>MSNQLFDAYFTAPAMREIFSDRGRLQGMLDFEAALARAEASAGLVPHSAVAAIEAACQAERYDTGALANAIATAGNSAIPLVKALGKVIATGVPEAERYVHLGATSQDAMDTGLVLQLRDALDLIEADLGKLADTLSQQALKHADTPLVGRTWLQHATPVTLGMKLAGVLGALTRHRQRLQELRPRLLVLQFGGASGSLAALGSKAMPVAEALAEQLKLTLPEQPWHTQRDRLVEFASVLGLVAGSLGKFGRDISLLMQTEAGEVFEPSAPGKGGSSTMPHKRNPVGAAVLIGAATRVPGLLSTLFAAMPQEHERSLGLWHAEWETLPDICCLVSGALRQAQVIAEGMEVDAARMRRNLDLTQGLVLAEAVSIVLAQRLGRDRAHHLLEQCCQRAVAEQRHLRAVLGDEPQVSAELSGEELDRL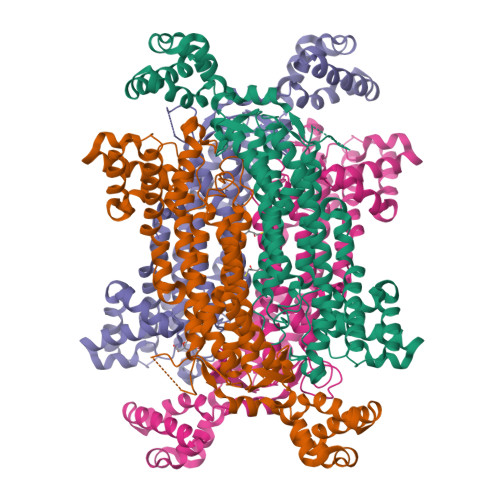LDPAHYLGQARVWVARAVSEHQRFTA[4x]>MARKLFTPITIKDMTLKNRIVMSPMCMYSSHEKDGKLTPFHMAHYISRAIGQVGLIIVEASAVNPQGRITDQDLGIWSDEHIEGFAKLTEQVKEQGSKIGIQLAHAGRKAELEGDIFAPSAIAFDEQSATPVEMSAEKVKETVQEFKQAAARAKEAGFDVIEIHAAHGYLIHEFLSPLSNHRTDEYGGSPENRYRFLREIIDEVKQVWDGPLFVRVSASDYTDKGLDIADHIGFAKWMKEQGVDLIDCSSGALVHADINVFPGYQVSFAEKIREQADMATGAVGMITDGSMAEEILQNGRADLIFIGRELLRDPFFARTAAKQLNTEIP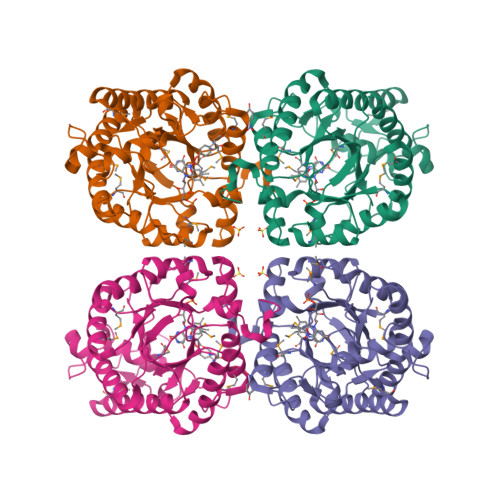APVQYERGW[2x]3H-PYRAZOLO[4,3-D]PYRIMIDIN-7-OL 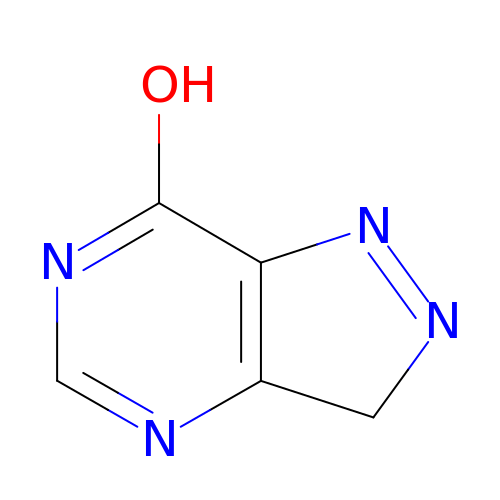| C5 H4 N4 O | OGCXIHWGXUQTCQ-UHFFFAOYSA-N The membrane protein Dispatched (Disp), which belongs to the RND family of small molecule transporters, is essential for Hedgehog (Hh) signaling, by catalyzing the extracellular release of palmitate- and cholesterol-modified Hh ligands from producing cells. Also uniquely among RND proteins, Disp activity requires Furin-mediated cleavage at a conserved site in its first large extracellular domain (ECD1), yielding a mature Disp protein consisting of two non-covalently associated fragments.

To further illuminate the mechanism of hDisp1-mediated Shh release, we generated a complex between hDisp1NNN and the native, dually lipidated Shh ligand, and subjected it to cryo-EM analysis. After the application of an adapted mask on ECDs and Shh for focused 3D classification, we solved the structure of the complex at an overall resolution of 4.07 Å. In the hDisp1NNN–Shh complex structure, the two ECDs of hDisp1 grasp Shh like a pincer, with the N-terminus of Shh facing upwards and close to ECD1 and the C-terminus of Shh facing downwards and close to the SSD. Upon Shh binding to hDisp1, Shh acts as a “molecular glue” that pulls the two ECDs of hDisp1NNN, turning them inwardly towards each other by approximately 4–5 Å. A comparison between the structures of hDisp1NNN-3C-cleaved and that of the hDisp1NNN–ShhN complex reveals conformational shifts of the two ECDs, whereas no substantial conformational change in the TMDs is observed. However, our structure reveals an extensive protein–protein interaction between hDisp1 and Shh. This interaction involves two interfaces, one primarily between residues 336–343 of ECD1 and residues 50–58 of Shh, and the other primarily between residues 242–249/260–265 of ECD1 and residues 68–81 of Shh. Resolution of the cryo-EM map at the hDisp1–Shh interface is approximately 4.5 Å, precluding analysis of the specific interacting residues. Although Shh was palmitate- and cholesterol-modified, we could not resolve the two lipid modifications, and thus any protein–lipid interactions between hDisp1 and Shh. Importantly, the Shh-binding site in hDisp1 clashes with the density corresponding to the uncleaved C-loop in the hDisp1NNN-3C structure, which provides an explanation for the drastically reduced Shh binding that we observed for uncleaved hDisp1NNN-3C.

> MAMSNGNNDFVVLSNSSIATSAANPSPLTPCDGDHAAQQLTPKEATRTKVSPNGCLQLNGTVKSSFLPLDNQRMPQMLPQCCHPCPYHHPLTSHSSHQECHPEAGPAAPSALASCCMQPHSEYSASLCPNHSPVYQTTCCLQPSPSFCLHHPWPDHFQHQPVQQHIANIRPSRPFKLPKSYAALIADWPVVVLGMCTMFIVVCALVGVLVPELPDFSDPLLGFEPRGTAIGQRLVTWNNMVKNTGYKATLANYPFKYADEQAKSHRDDRWSDDHYEREKREVDWNFHKDSFFCDVPSDRYSRVVFTSSGGETLWNLPAIKSMCNVDNSRIRSHPQFGDLCQRTTAASCCPSWTLGNYIAILNNRSSCQKIVERDVSHTLKLLRTCAKHYQNGTLGPDCWDMAARRKDQLKCTNVPRKCTKYNAVYQILHYLVDKDFMTPKTADYATPALKYSMLFSPTEKGESMMNIYLDNFENWNSSDGVTTITGIEFGIKHSLFQDYLLMDTVYPAIAIVIVLLVMCVYTKSMFITLMTMFAIISSLIVSYFLYRVVFHFEFFPFMNLTALIILVGIGANNAFVLCDVWNYTKFDKPHAETSETVSITLQHAALSMFVTSFTTAAAFYANYVSNITAIRCFGVYAGTAILVNYVLMVTWLPAVVVLHERYLLNIFTCFKKPQQQIYDNKSCWTVACQKCHKVLFAISEASRIFFEKVLPCIVIKFRYLWLFWFLALTVGGAYIVCINPKMKLPSLELSEFQVFRSSHPFERYDAEYKKLFMFERVHHGEELHMPITVIWGVSPEDNGNPLNPKSKGKLTLDSSFNIASPASQAWILHFCQKLRNQTFFYQTDEQDFTSCFIETFKQWMENQDCDEPALYPCCSHWSFPYKQEIFELCIKRAIMELERSTGYHLDSKTPGPRFDINDTIRAVVLEFQSTYLFTLAYEKMHQFYKEVDSWISSELSSAPEGLSNGWFVSNLEFYDLQDSLSDGTLIAMGLSVAVAFSVMLLTTWNIIISLYAIISIAGTIFVTVGSLVLLGWELNVLESVTISVAVGLSVNFAVHYGVAYRLAPDPDREGKVIFSLSRVGSAMAMAALTTFVAGAMMMPSTVLAYTQLGTFMMLIMCISWAFATFFFQCMCRCLGPQGTCGQIPLPKKLQCSAFSHALSTSPSDKGQSKTHTINAYHLDPRGPKSELEHEFYELEPLASHSCTAPEKTTYEETHICSEFFNSQAKNLGMPVHAAYNSELSKSTESDAGSALLQPPLEQHTVCHFFSLNQRCSCPDAYKHLNYGPHSCQQMGDCLCHQCSPTTSSFVQIQNGVAPLKATHQAVEGFVHPITHIHHCPCLQGRVKPAGMQNSLPRNFFLHPVQHIQAQEKIGKTNVHSLQRSIEEHLPKMAEPSSFVCRSTGSLLKTCCDPENKQRELCKNRDVSNLESSGGTENKAGGKVELSLSQTDASVNSEHFNQNEPKVLFNHLMGEAGCRSCPNNSQSCGRIVRVKCNSVDCQMPNMEANVPAVLTHSELSGESLLIKTL;> MLLLARCLLLVLVSSLLVCSGLACGPGRGFGKRRHPKKLTPLAYKQFIPNVAEKTLGASGRYEGKISRNSERFKELTPNYNPDIIFKDEENTGADRLMTQRCKDKLNALAISVMNQWPGVKLRVTEGWDEDGHHSEESLHYEGRAVDITTSDRDRSKYGMLARLAVEAGFDWVYYESKAHIHCSVKAENSVAAKSGGCFPGSATVHLEQGGTKLVKDLSPGDRVLAADDQGRLLYSDFLTFLDRDDGAKKVFYVIETREPRERLLLTAAHLLFVAPHNDSATGEPEASSGSGPPSGGALGPRALFASRVRPGQRVYVVAERDGDRRLLPAAVHSVTLSEEAAGAYAPLTAQGTILINRVLASCYAVIEEHSWAHRAFAPFRLAHALLAALAPARTDRGGDSGGGDRGGGGGRVALTAPGAADAPGAGATAGIHWYSQLLYQIGTWLLDSEALHPLGMAVKSS> MEDYTLREREQEIYNRQVIKRPFDPDSYLTADLHLYLKNGKTLTIHIERNLFFSHEFTWEEICRGAYREHYLSNSGPGKCDTQEYIDGLVADNGGRSTHNSSYLEPVAFQLTLLGNFDLGSIHLRIGDYLGFRDGQRFPCKETIHGRRDTIGPFMQGMSGKWAKEDYIHTYSGRFDCKTSRHPSIFLAFMRA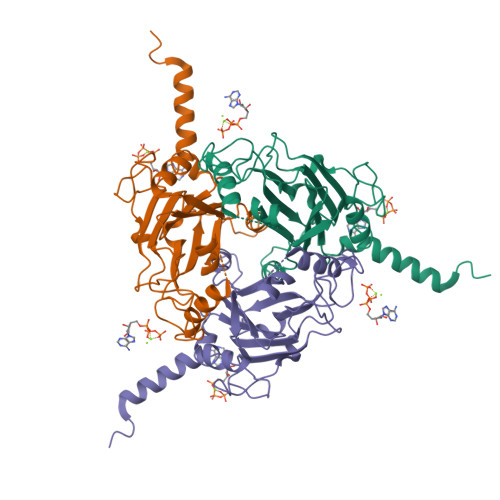NQDGHSSFAPENMRNALLYSGDKSPRYILMDNEHTLINNFIIPRCLPYRDQYGKDY> VQNDFLDSYDVTMLLQDDNGKQYYEYHKGLSLSDFEVLYGNTVDEIIKLRV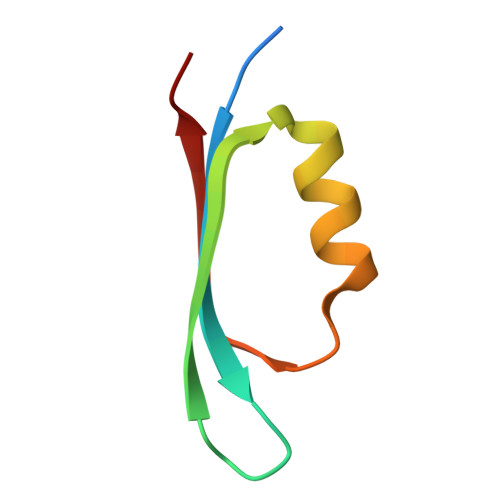DKIS>[2x]MAKKTSSKGKLPPYIFSPIPFLGHAIAFGKSPIEFLENAYEKYGPVFSFTMVGKTFTYLLGSDAAALLF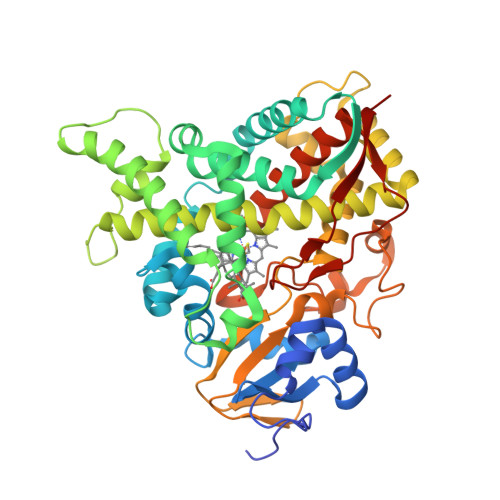NSKNEDLNAEDVYSRLTTPVFGKGVAYDVPNPVFLEQKKMLKSGLNIAHFKQHVSIIEKETKEYFESWGESGEKNVFEALSELIILTASHCLHGKEIRSQLNEKVAQLYADLAGGFSHAAWLLPGWLPLPSFRRRDRAHREIKDIFYKAIQKRRQSQEKIDDILQTLLDATYKDGRPLTDDEVAGMLIGLLLAGQATSSTTSAWMGFFLARDKTLQKKCYLEQKTVCGENLPPLTYDQLKDLNLLDRCIKETLRLRPPIMIMMRMARTPQTVAGYTIPPGHQVCVSPTVNQRLKDSWVERLDFNPDRYLQDNPASGEKFAYVPFGAGRHRCIGENFAYVQIKTIWSTMLRLYEFDLIDGYFPTVNYTTMIHTPENPVIRYKRRSK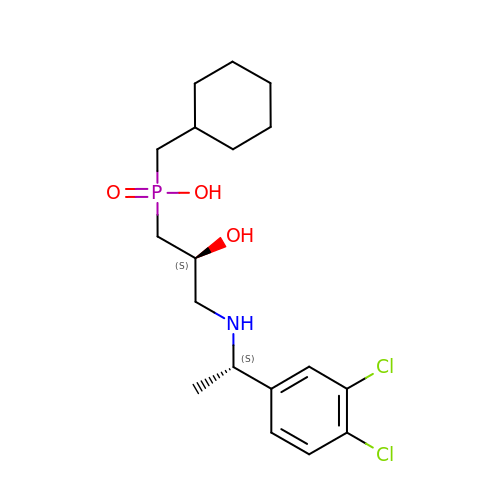(R)-(cyclohexylmethyl)[(2S)-3-{[(1S)-1-(3,4-dichlorophenyl)ethyl]amino}-2-hydroxypropyl]phosphinic acid | C18 H28 Cl2 N O3 P | JGGVBBYJRQOPPA-BBRMVZONSA-N>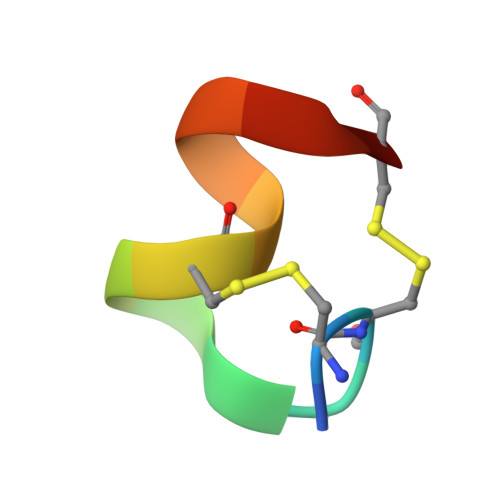 GCCSTPPCAVLYCX Here, we identify a PPi-dependent kinase belonging to the ribokinase family, which is distinct from the families of the previously reported PPi-dependent kinases. Accordingly, the phosphate donor specificity of TM0415 was investigated using myo-inositol as the acceptor. This analysis demonstrated that TM0415 utilizes PPi but neither ATP nor ADP to generate myo-inositol monophosphate. Structural comparison and sequence alignment with ATP-dependent or ADP-dependent members of the ribokinase family reveal the importance of five residues: two large hydrophobic residues occluding a part of the ATP-binding pocket and three basic residues specifically involved in PPi recognition. In general, the overall structure of the ribokinase family enzymes is divided into two domains: the phosphate-acceptor-binding domain (the N-terminal half) and the donor-binding domain (the C-terminal half).

In order to elucidate the PPi-binding mode of TM0415, we determined its crystal structure complexed with a PPi analog (methylenediphosphonic acid: PCP), which has a carbon atom instead of an oxygen atom in the bridge position of PPi. In an asymmetric unit, two protein molecules were found: chains A and B. Chain A was complexed with PCP, a magnesium ion, and myo-inositol, while chain B possessed a sulfate ion, which is derived from a crystallization precipitant, instead of PCP without any magnesium ions. The structures of chains A and B were very similar to each other (RMS distance 0.6 Å for 274 Cα atoms out of 275 chain B Cα atoms) and also similar to the unliganded structure (RMS distances 0.9 Å for 274 Cα atoms and 1.0 Å for 275 Cα atoms, respectively, out of 283 Cα atoms of the unliganded structure). In chain A, the phosphoryl group of PCP near myo-inositol (the proximal phosphoryl group) interacts with the main-chain nitrogen atoms of G231 and D234, while the other (the distal phosphoryl group) is surrounded by K171, T204, and R232. The two phosphoryl groups and four water molecules octahedrally coordinate with the magnesium ion, which is essential for the kinase activity. R229 is also located near PCP, but its side chain was disordered in the structure. The disorder of R229 in the PCP-complex structure is thought to result from the inability of the methylene group in PCP to form hydrogen bonds with the guanidine head of R229. D11, N78, Q141, and R145 in TM0415 interact with four of the six hydroxyl groups in myo-inositol, whereas D12, G26, Q136, R140, and D219 in MI3K_TK interact with all six hydroxyl groups. In the TM0415 structure, the probable catalytic residue D234 and the proximal phosphoryl group of PCP are nearest to the 1-hydroxyl group of myo-inositol (3.7 and 3.4 Å, respectively).

>MITFIGHVSKDVNVVDGKREIAYGGGVVMGAITSSLLGVKTKVITKCTREDVSKFSFLRDNGVEVVFLKSPRTTSIENRYGSDPDTRESFLISAADPFTESDLAFIEGEAVHINPLWYGEFPEDLIPVLRRKVMFLSADAQGFVRVPENEKLVYRDWEMKEKYLKYLDLFKVDSREAETLTGTNDLRESCRIIRSFGAKIILATHASGVIVFDGNFYEASFRSWSLEGRTGRGDTCTAAFLVGFVFKKMSIEKATKFAAAVTSVKMRHPGPLRREDLEAISGDQYF[2x]> GSHMASSAENEIEMRICDYLRRHGRSTVQDIFKELKLEKSTVNRHLYSLQASKQVFKTVEDNKRPVWNLVES

Unexpectedly, several fish species encode a PKR like kinase in which the two dsRNA-binding domains are substituted by two Z-DNA-binding Zalpha domains. PKZ interacts with CpG repeats, the DNA sequence that is more prone to adopt the left-handed helical conformation of Z-DNA. We expressed and purified the PKZ Zalpha domain (DrZalphaPKZ) encompassing residues 5–70 of zebrafish PKZ (DrPKZ). The protein was crystallized with an oligonucleotide forming a self-complementary (CG)6 DNA duplex with a single T base overhang and resulted in crystals belonging to two different space-groups growing under similar conditions.

The determination of both structures using molecular replacement revealed that the two crystal forms represent two different arrangements of protein molecules on the DNA helix due to the repeated nature of the DNA sequence. In the form that belongs to the tetragonal space-group I422 the two binding sites on the same DNA molecule are related with crystallographic symmetry resulting in the presence of just half the DNA segment in the asymmetric unit and the appearance of a continuous DNA helix throughout the crystal lattice. Overall, the two structures are superimposable in regard to their primary interactions with the nucleic acid and they mainly differ for the distribution of Zalpha molecules along the duplex. In both cases, four monomers are bound on the 12 bp duplex in agreement with the stoichiometry of the interaction deduced from gel-shift experiments where a protein/DNA ratio 4:1 is required for the complete shift (WT). Modeling of the alternative Zalpha arrangements on a long Z-DNA duplex shows that the 6 + 3 arrangement observed in the tetragonal form is the only that can propagate along a continuous helix without leading to protein-protein steric clashes as seen in the crystal structure. Based on the two structures, we created models of all possible arrangements, and we found that the tetragonal structure denoted as 6 + 3 represents the only arrangement of Zalpha domains that can propagate uniformly along a DNA helix without leading to protein–protein clashes. Although other arrangements may occur, as we see in different Zalpha crystal structures, the tetragonal arrangement is expected to settle at equilibrium with a long DNA helix. Based on this arrangement, we evaluated by modeling which of the possible pairs of Zalpha domains could represent the double Zalpha domain of PKZ, DAI and ADAR1, by being positioned in a way that they could satisfy constrains of a C-Terminus – N-terminus linkage between domains. We found that among the possible pairs one is topologically preferable, as it can accommodate a non-structured but geometrically possible poly-alanine linker, 15 residues long (two domain interactions).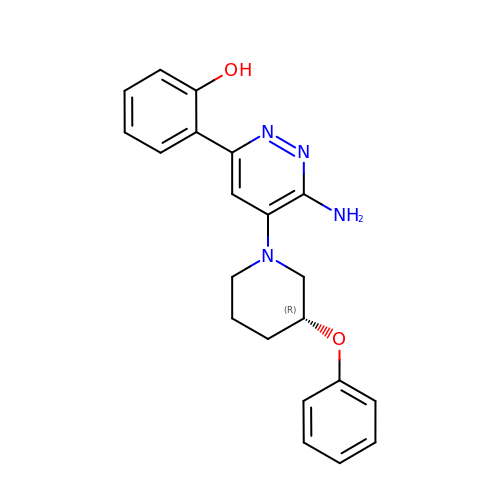2-[6-azanyl-5-[(3~{R})-3-phenoxypiperidin-1-yl]pyridazin-3-yl]phenol | C21 H22 N4 O2 | JOLHNCATQIAQLA-MRXNPFEDSA-N Multifunctional autoprocessing repeats-in-toxin (MARTX) toxins, secreted by multiple Gram-negative bacteria, are primary virulence factors that promote initial colonization, dissemination, and lethality in a wide range of hosts, including humans. By doing this, the clinical strain V. vulnificus MO6-24/O generates a MARTX toxin (MARTXVv) containing four effectors, which are arranged in the following order: domain of unknown function in the first position (DUF1), the Rho inactivation domain (RID), the α/β hydrolase domain (ABH), and a Makes caterpillars floppy-like effector (MCF) with a cysteine protease domain (CPD). Previously, we reported that DUF1 and RID within MARTXVv are not uncoupled by activated CPD in host cells; rather, they are discharged as a duet (it is assumed that the DUF1-RID effector module acts as a functional unit). The data show that DUF1 acts as a RID-dependent transforming NADase domain (RDTND) that disrupts NAD+ homeostasis by hijacking calmodulin.

Later, we did manage to generate crystals of DUF1-RIDCBD (residues, 1959–2374) in the absence of CaM, and determined the structure at a resolution of 3.38 Å. DUF1 within the DUF1-RIDCBD structure comprises the N-terminal domain (DUF1ND, residues 1959–2227), formed by a bundle of eight α helices (α1–α8), three 310 helices (310h1–310h3), and four short β strands (β1–β4), as well as a small lid domain (DUF1Lid, residues 2228–2264) formed by an α helix (α9), a 310 helix (310h4), and two short β strands (β5 and β6). RIDCBD composes three helices (α10−α12) and a mixed parallel and anti-parallel beta sheet (β7−β12). Of note, the two effectors are connected by α10, which forms part of the RIDCBD. Upon interaction with CaM, DUF1-RIDCBD undergoes a marked conformational change. Collectively, these data suggest that hijacking host CaM triggers marked rearrangement of the domains within DUF1-RIDCBD.

>GAMGEASHDSAESLVAARAEKVANLYRWLDTDNDVATDKYVPVPGFERVDVDVSDEVKQRMIQSMSGYIEHTDNQVPKDQAEALATLFVESTLDYDWDKRVEFLTKLESYGYSFEAPHAEKSIVSFWSGKNFKQYRDILDNAQTDGKKVVYDIDVKGNAFAIDLNKHLMRWGGLFLDPDNAEQNQLKSSIDAATFSNTGFWSSVYATGAQNDVYVIAEGGVRLGNYFWNVELPALRQLQREGLVGEIRLLDKPVSEYKDLPADQIGRRLTDAGVAVKVRFDALSHERQAELLADNPDGYKADTLVELDVKLSAIDSMLRESLPFYSLRTERNLLVQEGEEGFEVRSWPGIDGKSKTILLDNPEDAAQQKSIERFILANFDNFEQMPDELFLVDNKVLSHHDGRTRIIAQKEDGAWTYNT[2x]> GEIEFIESSKDAGFPVINTPSKTKLEPSVFHQVFEGNKEPAVLRSGDPRLKANFEEAIFSKYIGNVNTHVDEYMLEAVDHYAGQLATLDISTEPMKLEDAVYGTEGLEALDLTTSAGYPYVALGIKKRDILSKKTKDLTKLKECMDKYGLNLPMVTYVKDELRSIEKVAKGKSRLIEASSLNDSVAMRQTFGNLYKTFHLNPGVVTGSAVGCDPDLFWSKIPVMLDGHLIALDYSGYDASLSPVWFACLKMILEKLGYTHKETNYIDYLCNSHHLYRDKHYFVRGGMPSGCSGTSIFNSMINNIIIRTLMLKVYKGIDLDQFRMIAYGDDVIASYPWPIDASLLAEAGKGYGLIMTPADKGECFNEVTWTNVTFLKRYFRADEQYPFLVHPVMPMKDIHESIRWTKDPKNTQDHVRSLCLLAWHNGEHEYEEFIRKIRSVPVG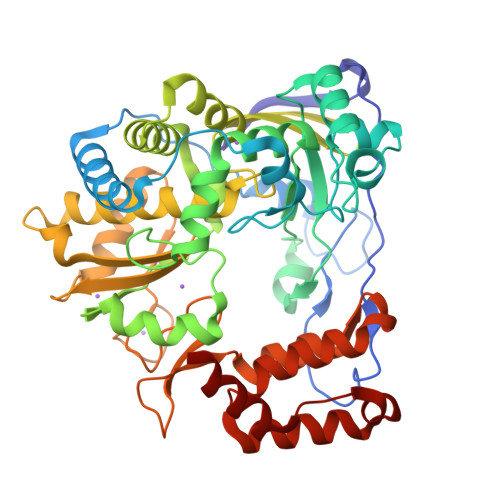RCLTLPAFSTLRRKWLDSF> AQTHALSNAAVMDLQSRWENMPSTEQQDIVSKLSERQKLPWAQLTEPEKQAVWYISYGEWGPRRPVLNKGDSSFIAKGVAAGLLFSVGLFAVVRMAGGQDAKTMNKEWQLKSDEYLKSKNA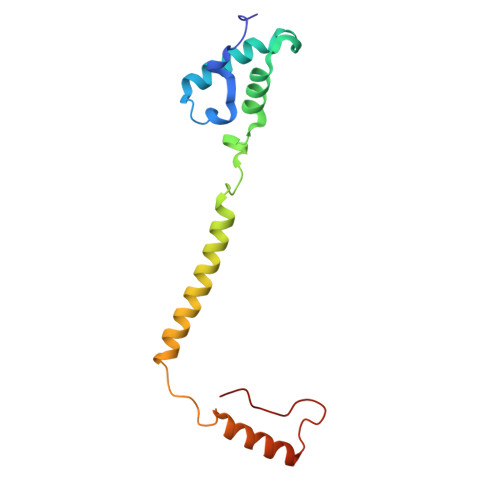NPWGGYSQVQSK DNA-stabilized silver nanoclusters (DNA-AgNCs) are emissive systems comprising a small aggregate of silver atoms and cations wrapped in one or multiple DNA strands. The Ag16NC is embedded in two 10-base oligomers (5′-CACCTAGCGA-3′), containing two guanosines. We therefore designed three inosine (I) mutants: I7 (5′-CACCTAICGA-3′) and I9 (5′-CACCTAGCIA-3′), where the guanosine in position 7 and 9 was replaced respectively, and I7–I9 (5′-CACCTAICIA-3′) where both guanosines were substituted. Single crystal X-ray diffraction measurements unravelled the structure of the I7 and I7–I9 mutants, allowing us to understand how the observed spectroscopic changes are related to the amino groups in position 7 and 9.

While we were unable to determine the structure of the I9 mutant, we managed to crystallize and resolve the structure of the I7–I9 double mutant. Therefore, we used the structural information obtained from the I7–I9_DNA-Ag16NC crystal around position 9 and assumed that it can provide a reasonable picture of the spectroscopic behavior of the I9 mutant. Since the I9 and C4 nucleotides are directly bound to the Ag16NC, the absence of these possible interactions might be less relevant or even not relevant at all. Note that there are six I7–I9_DNA-Ag16NCs in the asymmetric unit cell of the I7–I9 mutant (see Fig. S23†) with O6(I9)–N4(C4) distances spanning from 2.5 to 3.2 Å. Additional stabilization is ensured by hydrogen bonds between G9 and C4, particularly between O6 (G9) and the exocyclic N4 (C4) and potentially between N2 (G9) and O2 (C4), although the latter distances are larger (2.9–3.3 Å).10 Consequently, when G9 is replaced by I9, the two potential hydrogen bonds between N2(G9)–O2(C4) are missing. When both positions are substituted, an average decay time of 4.09 ns is found, which is similar to I9. Fig. S9† shows that hydrogen bonding interactions are still possible between I7 and T5, making the absence of the amino group in I9 the dominant effect. Note that the low occupancy silver cation bound to I7, seen in the I7 mutant, is now absent. Interestingly, the doubly substituted mutant had spectroscopic features more similar to the I9 mutation, with respect to <τw>, while it was more alike to the I7 mutant in relation to <τμs>.

>CACCTAICIA[12x]>[3x]MPLDAGGQNSTQMVLAPGASIFRCRQCGQTISRRDWLLPMGGDHEHVVFNPAGMIFRVWCFSLAQGLRLIGAPSGEFSWFKGYDWTIALCGQCGSHLGWHYEGGSQPQTFFGLIKDRLAEGP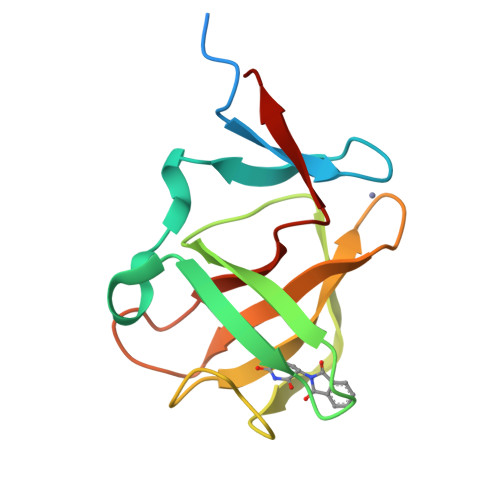AD;> KFFEQMQQ>MAEELVLERCDLELETNGRDHHTADLCREKLVVRRGQPFWLTLHFEGRNYEASVDSLTFSVVTGPAPSQEAGTKARFPLRDAVEEGDWTATVVDQQDCTLSLQLTTPANAPIGLYRLSLEASTGYQGSSFVLGHFILLFNAWCPADAVYLDSEEERQEYVLTQQGFIYQGSAKFIKNIPWNFGQFEDGILDICLILLDVNPKFLKNAGRDCSRRSSPVYVGRVVSGMVNCNDDQGVLLGRWDNNYGDGVSPMSWIGSVDILRRWKNHGCQRVKYGQCWVFAAVACTVLRCLGIPTRVVTNYNSAHDQNSNLLIEYFRNEFGEIQGDKSEMIWNFHCWVESWMTRPDLQPGYEGWQALDPTPQEKSEGTYCCGPVPVRAIKEGDLSTKYDAPFVFAEVNADVVDWIQQDDGSVHKSINRSLIVGLKISTKSVGRDEREDITHTYKYPEGSSEEREAFTRANHLNKLAEKEETGMAMRIRVGQSMNMGSDFDVFAHITNNTAEEYVCRLLLCARTVSYNGILGPECGTKYLLNLNLEPFSEKSVPLCILYEKYRDCLTESNLIKVRALLVEPVINSYLLAERDLYLENPEIK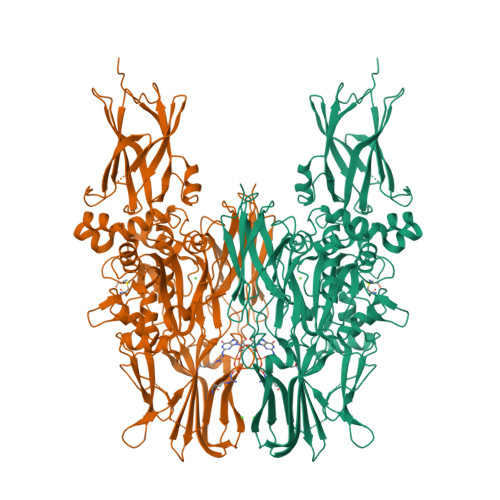IRILGEPKQKRKLVAEVSLQNPLPVALEGCTFTVEGAGLTEEQKTVEIPDPVEAGEEVKVRMDLLPLHMGLHKLVVNFESDKLKAVKGFRNVIIGPA[3x]> GSMENTDVFLGLHDFLERMRKPSAGDFVKSIKSFIVSFSNNAPDPEKDCAMVQEFF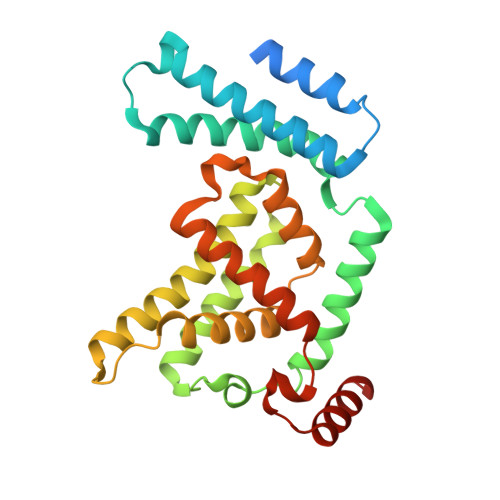SKMEAAFRAHPLWSGCSEEELDSAGDGLEKYVMTKLFTRVFASNTEEVIADEKLFQKMSLVQQFISPENLDIQPTFQNESSWLLAQKELQKINMYKAPRDKLVCILNCCKVINNLLLNASIASNENAPGADEFLPVLIYVTIKANPPQLHSNLLYIQRYRRESKLVGEAAYFFTNILSAESFISNIDAKSISLDEAEFEKNMESARARISG> MEVYVPPPRVMAPTEGRNSISYNPIAPLQDTTHIYIIDNKTSDIENLNIHKDHSNFYTNIVQNVDVAPSDAATQTIKLDERSRWGGELHTILKTNAPNVTEFFNSNSFKALLMSDKTDPANPVYTWFELSIPEGDYTVGSLIDMLNNAVVENYLEVGRQKGVQISDIGVKFDTRNFSLGRDPLTSLVTPGNYTFKAFHPDIVLLPGCGVDFTHSRINNMLGMRKRFPYEPGYVITYEDLVGGNIPALLDLAKYPGETSPVLQDPDGNSYHVEE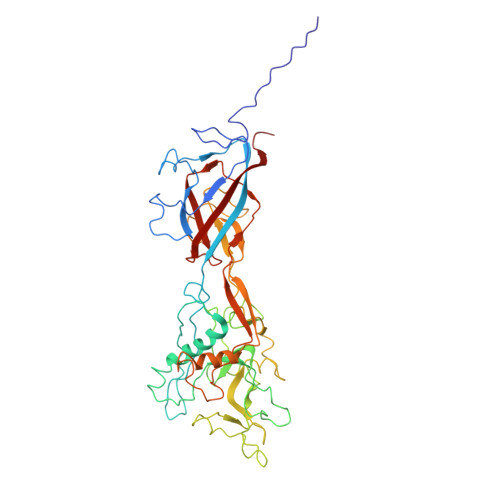VSPKKWQTKYRSWCLAYNSSQGTLKSEQILTVPDITGGLGQLYWSLPDAFKPPVTFTNNTTDISTQPVTGMHLFPLSQRIVYNTSAVYAQLVEQMTNNTKVFNRFPKNAILMQPPYDTTQWISENVPYVADHGIQPLKNSLTGVQRVTLTDDRRRSCPYIYKTLATVTPKVLSSATLQ>MSKIRIGIVGYGNLGRGVEAAIQQNPDMELVAVFTRRDPKTVAVKSNVKVLHVDDAQSYKDEIDVMILCGGSATDLPEQGPYFAQYFNTIDSFDTHARIPDYFDAVNAAAEQSGKVAIISVGWDPGLFSLNRLLGEVVLPVGNTYTFWGKGVSLGHSGAIRRIQGVKNAVQYIIPIDEAVNRVRSGENPELSTREKHAMECFVVLEEGADPAKVEHEIKTMPNYFDEYDTTVHFISEEELKQNHSGMPNGGFVIRSGKSDEGHKQIIEFSLNLESNPMFTSSALVAYARAAYRLSQNGDKGAKTVFDIPFGLLSPKSPEDLRKE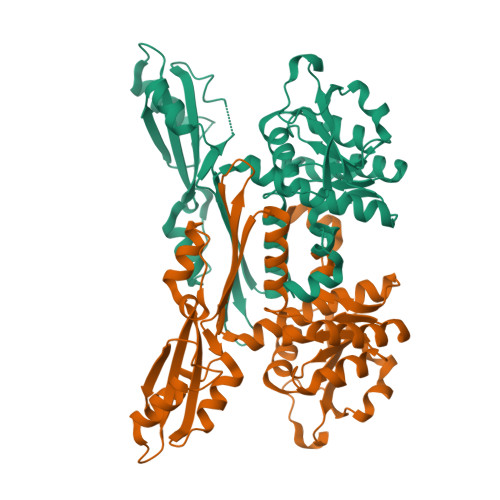LL[2x]> GAMSGGLLKALRSDSYVELSQYRDQHFRGDNEEQEKLLKKSCTLYVGNLSFYTTEE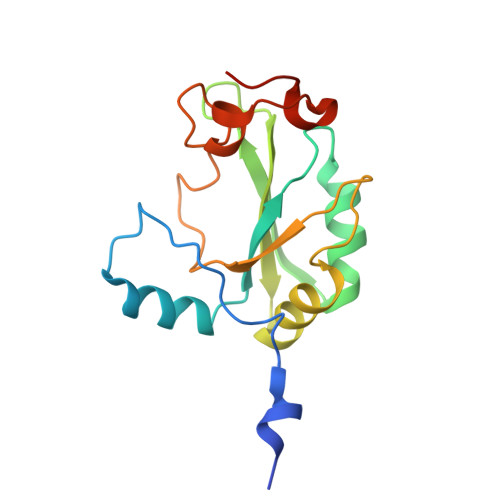QIYELFSKSGDIKKIIMGLDKMKKTACGFCFVEYYSRADAENAMRYINGTRLDDRIIRTDWDAGFKEGRQYGRGRSGGQVRDEYRQDYDAGRGGYGKLAQNQ>[2x]GIDPFTTARKSTGGKAPRKGGMVVKKRKLATEAGGSDERPKYLPGKHPKNQEKT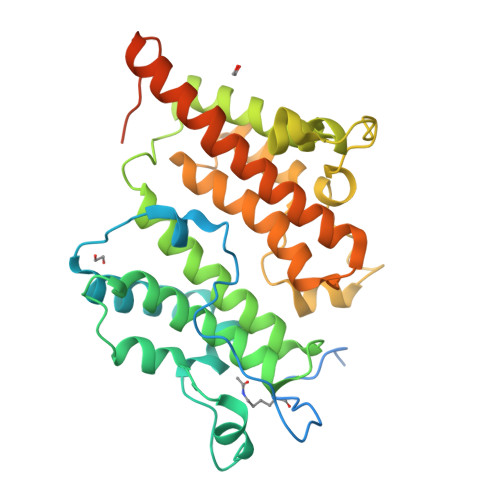PHVDYNAPLNPKSELFLDDWHIPKFNRFISFTLDVLIDKYKDIFKDFIKLPSRKFHPQYYYKIQQPMSINEIKSRDYEYEDGPSNFLLDVELLTKNCQAYNEYDSLIVKNSMQVVMLIEFEVLKAKNLKRNYLINSEVKAKLLHYLNKLVDATEKKINQALLGASSPKNLDDKVKLSEPFMELVDKDELPEYYEIVHSPMALSIVKQNLEIGQYSKIYDFIIDMLLVFQNAHIFNDPSALIYKDATTLTNYFNYLIQKEFFPELQDLNERGEINLEFDKFEFENYLAIGGGGPAAAGALAISALDND>MNMIDQLNITDFQVFTDENS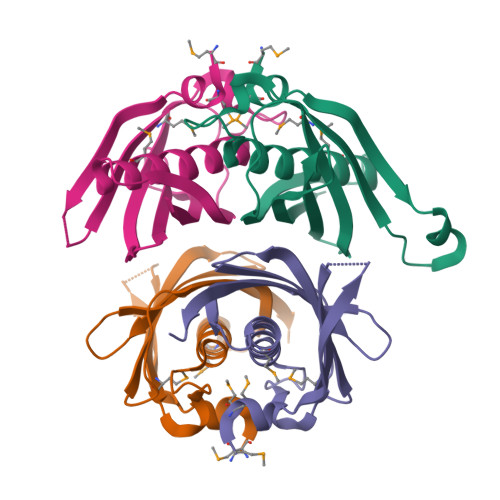DKFVSKIYKFSSKMILSDFHAQPQGFLNGGASLALAEITAGMASNAIGSGQYFAFGQSINANHLNPKKCEGFVNARGLLLKNGKRNHVWEIKITDENETLISQITVVNALVPQKNSDKLEHHHHHH[4x]Bacterial enhancer binding proteins (bEBPs) are specialized AAA+ proteins that are required to activate the sigma54-dependent transcriptional complexes. As transcriptional activators, bEBPs function to catalyze the conversion of RPc to RPo, causing the RNAP-σ54 holoenzyme to isomerize and promoter DNA to melt, leading to transcription initiation. The ‘Glutamate Switch’ pair (E-N) was identified originally in PspF as the E108 side chain adopts different conformations in the presence of ATP or ADP, forming or interrupting the interactions with N64 (3,11,16,22,27). In order to understand the biochemical properties of E108Q and to provide a structural basis for the ‘Glutamate Switch’ pair, we determined the crystal structures of E108Q mutant of PspF AAA+ domain (PspF1–275E108Q) in the absence of nucleotide (APO), and in the presence of Mg-ATP or Mg-ADP.

The crystals diffracted to 1.6–1.8 Å and have the same space group and unit cells as those of WT proteins and are thus subsequently rebuilt and refined using WT protein structures as templates. We first compared the conformations surrounding the ‘Glutamate Switch’. In WT protein, when ADP is bound, E108 does not interact with N64 albeit in the ATP bound or APO state, E108 interacts with N64 (Figure 6A, (16)). In the mutant structures, on the contrary, E108Q in the ADP bound state as well as in the APO state also interacts with N64. This conformation, which enables the ‘Glutamate Switch’ pair to interact, is linked to the ability of PspF being able to engage with its target, the RPc. The crystal structures of the E108Q therefore suggest that PspF E108Q variant could engage with RPc, irrespective of its nucleotide bound states. Such a conformation could contribute to the ability of E108Q to bind RPc and move RPc along the pathway of transcription activation despite its slow ATPase activity. E108Q, on the other hand, is hexameric irrespective of the nucleotide being present, suggesting that the reduced ATPase activity is due to a reduced hydrolysis reaction per se, and not due to gross defects in hexamerisation nor loss of nucleotide binding.

> MAEYKDNLLGEANSFLEVLEQVSHLAPLDKPVLIIGERGTGKELIASRLHYLSSRWQGPFISLNCAALNENLLDSELFGHEAGAFTGAQKRHPGRFERADGGTLFLDQLATAPMMVQEKLLRVIEYGELERVGGSQPLQVNVRLVCATNADLPAMVNEGTFRADLLDRLAFDVVQLPPLRERESDIMLMAEYFAIQMCREIKLPLFPGFTERARETLLNYRWPGNIRELKNVVERSVYRHGTSDYPLDDIIIDPFKRRPPEDAIA> MAEEQQNSDQSNGGNVIPTPEEVATFLHKTVEEGGWEKCWEEEITPWDQGRATPLIVHLVDTSSLPLGRALVPGCGGGHDVVAMASPERFVVGLDISESALAKANETYGSSPKAEYFSFVKEDVFTWRPTELFDLIFDYVFFCAIEPEMRPAWAKSMYELLKPDGELITLMYPITDHVGGPPYKVDVSTFEEVLV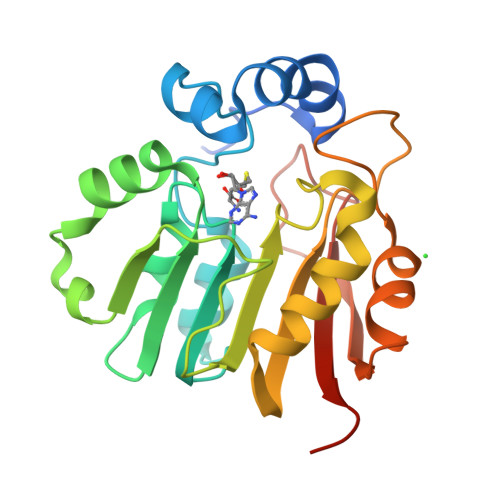PIGFKAVSVEENPHAIPTRKGKEKLGRWKKINLEHHHHHH>[2x]MRGSHHHHHHENLYFQGSMLIDLITSCRKSTVIYAFVDMGLSVHFKDGACVNISELASQYGLDHSRFSRLCEYLIKIGVLVSCNEGVALSEECSALADPESMESLMIRCEVSPEYWKAWSMYSKSLYENNSKTAFEIAHGKPFFEYLDHHELFRSNFDSFMSKNSDKIIEKLLDIYDFSQHNRILDVGGGEGNLLIRINEKIKGKHYAV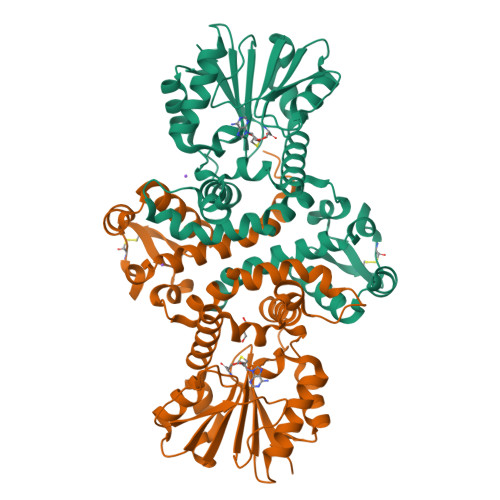LDRYNETPVLEDIEFINGDFFKLVPSGYDLYILKNVIHNWSDSNAILILENCRKAMDDNATILLIGTVKKLKLEIIDSTDILMDVLLLGKERYLNELEDLAHQAGFVVKDIKEINEKYSIIELGVK> MEANGLGPQGFPELKNDTFLRAAWGEETDYTPVWCMRQAGRYLPEFRETRAAQDFFSTCRSPEACCELTLQPLRRFPLDAAI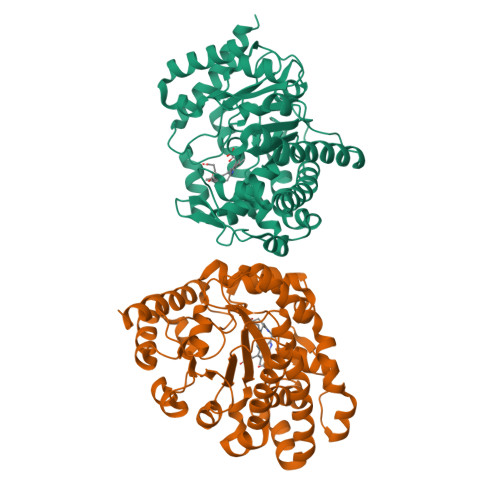IFSDILVVPQALGMEVTMVPGKGPSFPEPLREEQDLERLRDPEVVASELGYVFQAITLTRQRLAGRVPLIGFAGAPWTLMTFMVEGGGSSTMAQAKRWLYQRPQASHQLLRILTDALVPYLVGQVVAGAQALQLFESHAGHLGPQLFNKFALPYIRDVAKQVKARLREAGLAPVPMIIFAKDGHFALEELAQAGYEVVGLDWTVAPKKARECVGKTVTLQGNLDPCALYASEEEIGQLVKQMLDDFGPHRYIANLGHGLYPDMDPEHVGAFVDAVHKHSRLLRQN>[2x]GGSDDARTSIEQRSNAVSQVLLGIFS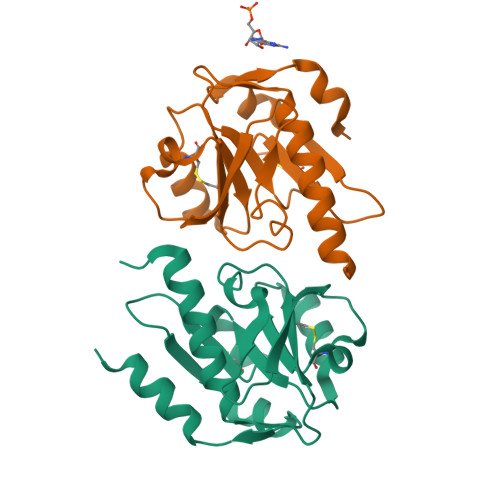YVRWPKEPAVLQLCVVGPTEYADGLLRGMVQANGRRVHAERRAVDNPDLGTLCNVIYLGVVDERERQQVFRSLAGHPVLSISERGTECSVGSMFCLNVGGPRITFEANLDSIARSGVRVHPSVLKLARRQATP4-{[2-(2-hydroxyphenyl)imidazo[1,2-a]pyrazin-3-yl]amino}benzene-1,2-dicarboxylic acid 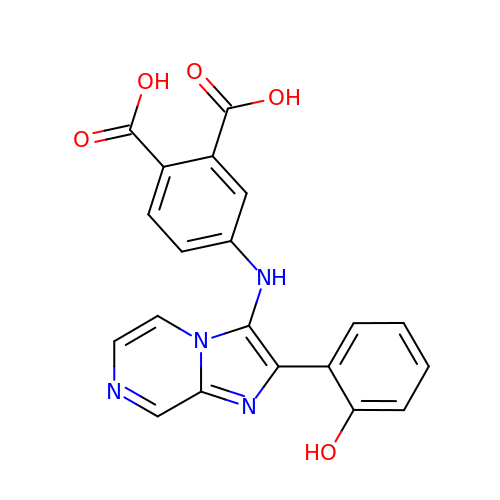| C20 H14 N4 O5 | XBODYKBLJPPTJV-UHFFFAOYSA-N> SMRVKNLKSRLRGGKMRYQEEEARLASFRNWPFYVQGISP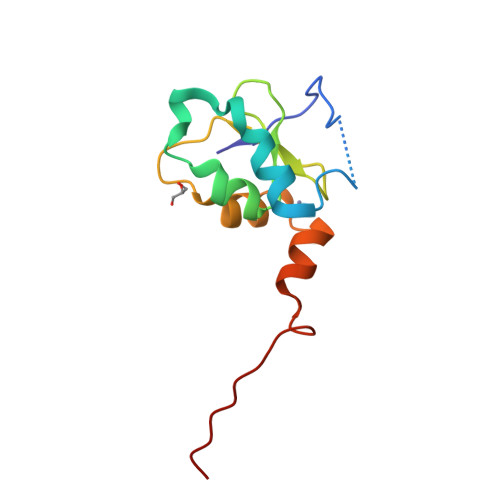CVLSEAGFVFTGKQDTVQCFSCGGCLGNWEEGDDPWKEHAKWFPKCEFLRSKKSSEEITQYIQSYK> MHHHHHHHHENLYFQGSETPAEPKPPVVVEAHQVDTFDVPGVFYENHPHEPHLSGMNEYNQLYQQSINDPDTFWARMARDLITFEKDFDKTHIGTLEGGDNAWFVGGRLNASFNCVDRHAMRDPNKVAIIYEADEPGHGRSITYAELLKEVSRLAWVMKSQGVRRGDTVAIYLPMIPEAIFALLACARIGAIHSVVFAGFSSDSLRDRTLDARSKFIITTDEGKRGGKVIGTKKIVDEALKQCPDVTS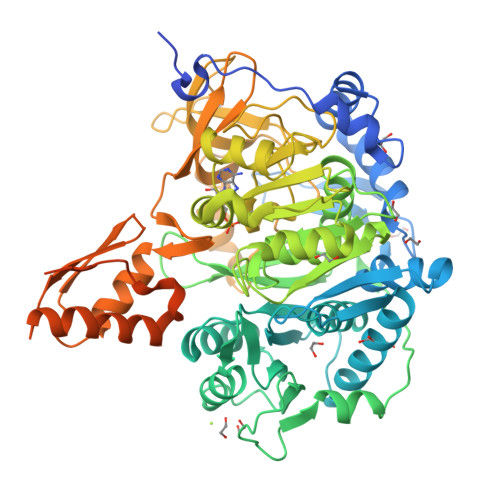CLVFKRTGADVPWTKGRDLWWHEEVEKYPNYLPAESMDSEDPLFLLYTSGSTGKPKGVMHTTAGYLVGAAATGKYVFDIHPADRFFCGGDVGWITGHTYVVYAPLLLGCTTVVFESTPAYPNFSRYWDVIEKHKVTQFYVAPTALRLLKRAGDHHINHEMKDLRILGSVGEPIAAEVWKWYHEVVGKRQAHIVDTYWQTETGSHVITPLGGITPTKPGSASLPFFGIDPVILDPVTGAEIPGNDVEGILAFRKPWPSMARTVWGDHKRYMDTYLNVYKGFYFTGDGAGRDHEGYYWIRGRVDDVVNVSGHRLSTAEIEAALIEHHCVAEAAVVGVPDPLTGQAVHAFVALKSGNDNREQLRKELIMQVRKSIGPFAAPKVVFVIDDLPKTRSGKIMRRILRKILSGEEDSLGDISTLSDPSVVNKIIDTFHEWKRAMAAAAAAAAAVSATAPPNSTTG>[2x]SNAMALGFGMKMELQQFLDALASSPEKIEFETTMAVIEDNYDFTPAAFTNGNTQNDANENNGSCKIFAFGLLNALDKEATLACFGRFYREDV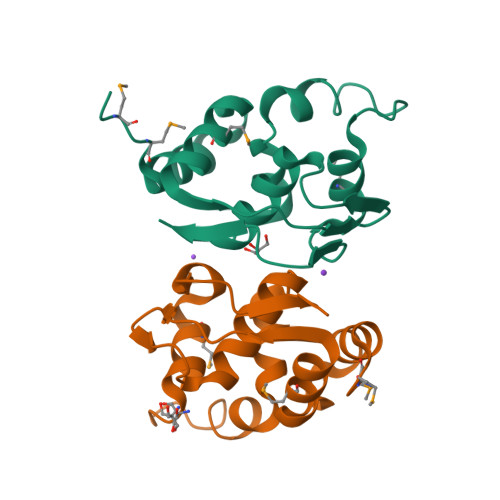LLHPENNDHQNIRNFMVTGWEGIQFETSALTAK>[2x]HHHHHHSQDPMSNTADFRLQTSTLCHSFLLASANKQDTDYLTDLLDNTNIDLTCVP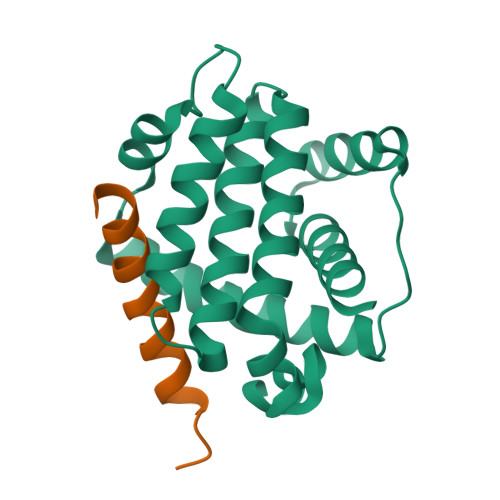NGQEIIHSLLQLVGDFNQRFSQTHEIEPVAQSLGIDSDKPVDKTALEIFYLEILNGLFEKLNWGRIVAMFAFLRILVLRLSKHGHSDAIQMLIKTTSQYSDEKLKNWINLHDGWSGLIEFSGR;>LPLQPSSTMGQVGRQLAIIGDDINRRYDSEFQTM[2x]>MAHHHHHHMTSTATSSPRVITSSPVVVALDYDNRDKALAFVERIDPRDCRLKVGKEMFTLLGPQFVRDLHQRGFEVFLDLKFHDIPNTTARAVAAAAELGVWMVNVHASGGARMMTAA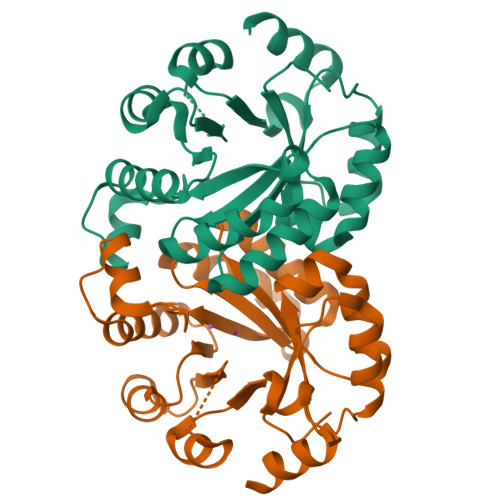REALLPFGKEAPLLIAVTVLTSMEASDLQDLGIMLSPADHAAKLAALTKRCGLDGVVCSAQEAVRFKQELGQEFKLVTPGIRPTGSDAGDQRRIMTPEQAQQAGVDYMVIGRPVTQSADPVATLASINASLNKGV[8x]>APTAPMTNPDSGVVVGYWHNWCDGGGYQGGNAPCVTLDEVNPMYNIVNVSFMKVYDVADGRIPTFKLDPTIGLSEEQFIDQISELNKQGRSVLLALGGADAHVELETGDERAFADEIIRLTERYGFDGLDIDLEQAAVTAANNQTVIPDALKLVKDHYRAEGKNFLITMAPEFPYLTTGGKYVPYIDNLEGYYDWINPQFYNQGGDGIWVDGVGWIAQNNDALKEEFIYYISDSLINGTRGFHKIPHDKLVFGIPSSIDAAATGFVQDPQDLYDAFETLTTQGQPLRGVMTWSINWDMGTNKNGQQYNEQFIKDYGPFVHGQVTPPPVLEHHHHH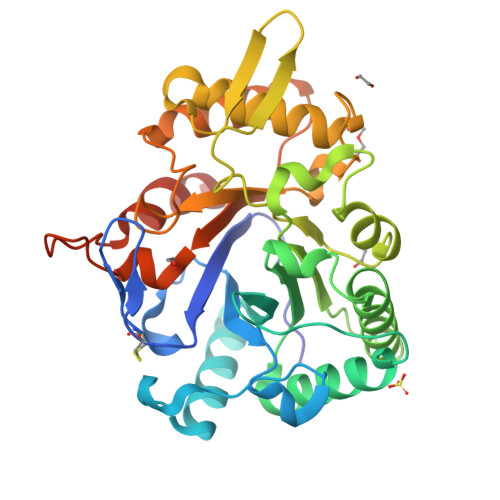H[6x]>[15x]SADVAGAVIDGAGLGFDVLKTVLEALGNVKRKIAVGIDNESG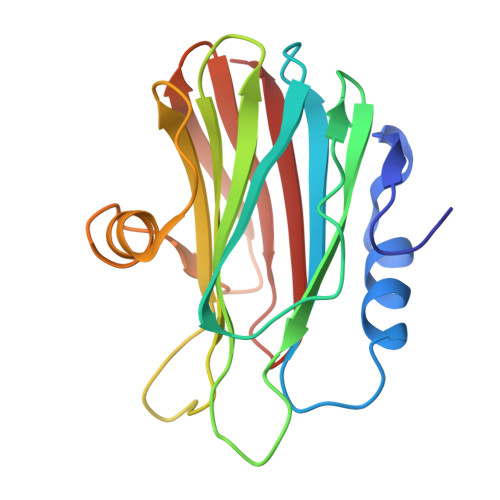KTWTAMNTYFRSGTSDIVLPHKVAHGKALLYNGQKNRGPVATGVVGVIAYSMSDGNTLAVLFSVPYDYNWYSNWWNVRVYKGQKRADQRMYEELYYHRSPFRGDNGWHSRGLGYGLKSRGFMNSSGHAILEIHVTKA> ADNLAEFHVQNQECDSCHTPDGELSNDSLTYENTQCVSCHGTLAEVAETTKHEHYNAHASAFPGEVACTSCHSAHEKSMVYCDSCHSFDFNMPYAKKWLRDEPTIAELAKDKSERQAALASAPHDTVDVVVVGSGGAGFSAAISATDSGAKVILIEKEPVIGGNAKLAAGGMNAAWTDQQKAKKITDSPELMFEDTMKGGQNINDPALVKVLSSHSKDSVDWMTAMGADLTDVGMMGGASVNRAHRPTGGAGVGAHVVQVLYDNAVKRNIDLRMNTRGIEV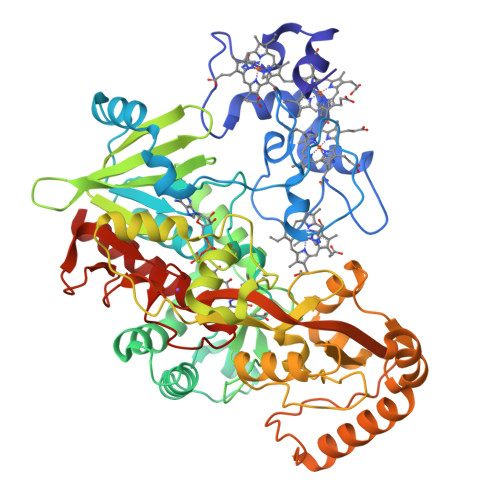LKDDKGTVKGILVKGMYKGYYWVKADAVILATGGFAKNNERVAKLDPSLKGFISTNQPGAVGDGLDVAENAGGALKDMQYIQAHPTLSVKGGVMVTEAVRGNGAILVNREGKRFVNEITTRDKASAAILAQTGKSAYLIFDDSVRKSLSKIDKYIGLGVAPTADSLVKLGKMEGIDGKALTETVARYNSLVSSGKDTDFERPNLPRALNEGNYYAIEVTPGVHHTMGGVMIDTKAEVMNAKKQVIPGLYGAGEVTGGVHGANRLGGNAISDIITFGRLAGEEAAKYSKKN>[3x]NKGSIEGREPAVYFKEQFLDGDGWTSRWIESKHKSDFGKFVLSSGKFYGDEEKDKGLQTSQDARFYALSASFEPFSNKGQTLVVQFTVKHEQNIDCGGGYVKLFPNSLDQTDMHGDSEYNIMFGPDICGPGTKKVHVIFNYKGKNVLINKDIRCKDDEFTHLYTLIVRPDNTYEVKIDNSQVESGSLEDDWDFLPGSGDPSIYAYDNFGVLGLDLWQVKSGTIFDNFLITNDEAYAEEFGNETWGVTKAAEKQMKDKQDEEQRLK

shown to play a key role in the MHC class I assembly pathway. cellular processes with broad patho-physiological implications. GSG linker and the C-terminal residues 369–417 were deleted. The long C-terminal α3 helix is kinked at Thr346.

to two different crystal forms in our study. yielded similar structures, except for their N-terminal extension. end of α3 between different molecules of the first crystal form. interactions were observed in the first crystal form. mode observed in the first crystal form.>RDLEAAYNNLLRDKSALEEEKRQLEQENEDLARRLESS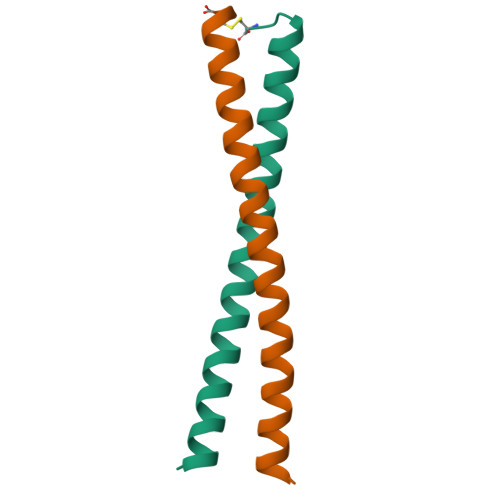SEEVTRLRRGQC[4x]>[4x]MEADARSIYVGNVDYGATAEELEAHFHGCGSVNRVTILCDKFSG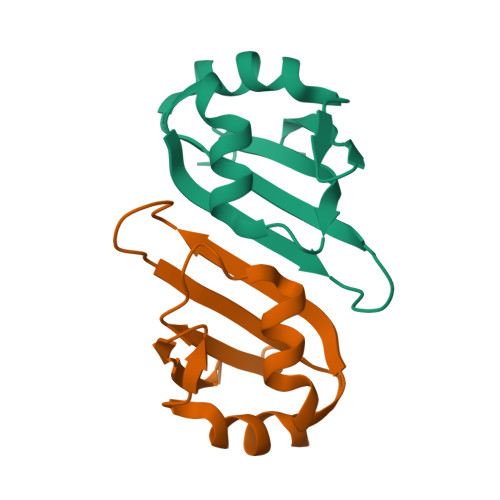HPKGFAYIEFSDKESVRTSLALDESLFRGRQIKVIPKRTNRPGILEHHHHHH> GHMDEISETNTIFKLEGVSVLSPLRKKLDLVFYLSNVDGSPVITLLKGNDRELSIYQLNKNIKMASFLPVPEKPNLIYLFMTYTSCEDNKFSEPVVMTLNKENTLNQFKKLGLLDSNVTDFEKCVEYIRKQAILTGFKISNPFVNSTLVDTDAEKINSFHLQCHRGTKEGTLYFLPDHIIFGFKKPILLFDASDIESI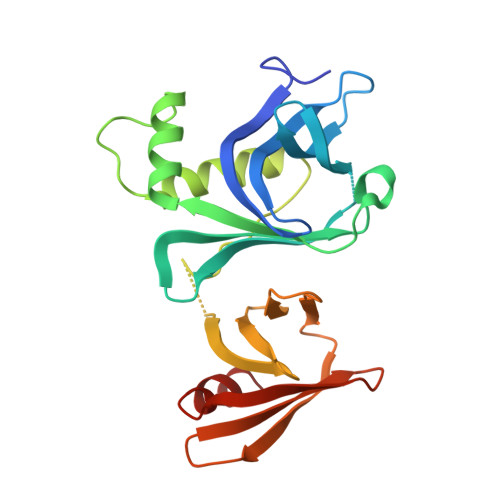TYSSITRLTFNASLVTKDGEKYEFSMIDQTEYAKIDDYVKRK> RLLGAPVPVDENDEGLQRALQFAMAEYNRASNDKYSSRVVRVISAKRQLVSGIKYILQVEIGRTTCPKSSGDLQSCEFHDEPEMAKYTTCTFVVYSIPWLNQIK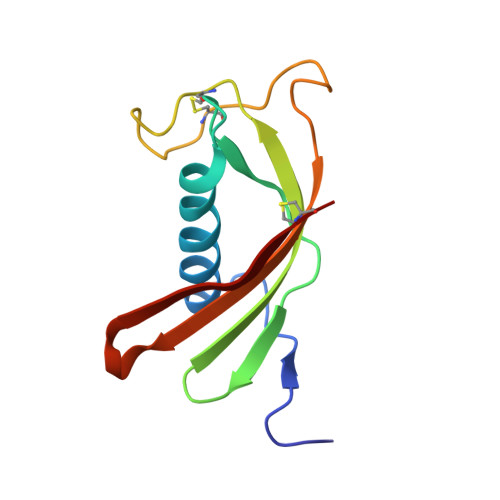LLESKCQ Inositol 1,3,4,5,6-pentakisphosphate 2-kinase (IP5 2-K)3 is a key enzyme of higher inositol phosphate (inositide, IP) metabolism. IP5 2-K is present in yeast to mammals and catalyzes the synthesis of phytic acid (inositol hexakisphosphate or IP6) from IP5 and ATP. Mouse IP5 2-K folds in two lobes, N- and C-terminal lobes, connected by a hinge, thereby conserving the general fold scheme of PKs and IPKs, and in a similar way, both lobes coordinate the nucleotide between them. The CIP lobe represents more than half of the protein and is specific to IP5 2-K enzymes.

We have solved the structure of Mus musculus IP5 2-K (mIP5 2-K) at 2.4 Å resolution from a truncated form lacking the 21 C-terminal residues (ΔC-mIP5 2-K). In addition, we present two different crystal forms, including one or two molecules in the asymmetric unit, respectively, the first showing much better resolution (2.4 versus 3.2 Å). Unexpectedly, the formation of the ternary complex (mIP5 2-K + IP5 + ATP) was achieved by protein incubation with IP6 and ADP. The triphosphate moiety is tightly bound to the N-lobe of the enzyme through polar interactions and to the C-lobe through two magnesium ions. Regarding the inositide substrate, IP5 is tightly bound to the enzyme through its five phosphates. Residues Lys-138 and Asp-400 make direct interaction with Pγ and/or the nucleophile 2-OH. The distance between the 2-OH and Pγ oxygen is 3.2 Å suggesting an in-line transference mechanism probably in agreement with an associative mechanism. Pγ is oriented through a magnesium ion (Mg1) coordinated to Asp-437 and to Asp-439 in a second sphere. Asp-437 also coordinates a second magnesium ion (Mg2) together with Ser-402 through a water molecule. The Zn1 site is formed by residues from two CIP lobe elements: Cys-159, Cys-162, and Cys-181 from CIP-I and Cys-291 from CIP-II.

> GEFMEEGKMDENEWSYHGEGNKSLVVAHAQRCVVLRFLKFPPNKKKTSEEILQHLQNIVDFGKNVMKDFLGENYVHCGEVVQLPLEFVKQLCLKIQCERPESRCDKDLDTFSGYAMCLPNLTRLQTFHFAEHRPILCVEIKPKCGFIPFSNDVTHEMKHKVCRYCMHQHLKVATGKWKKISKYCPLDLYSGNKQRMHFALRSLLQETQNNLRIFKNGELIYGCGDARSPVADLKELAHHLKPFFFPSNGLASGPHCTKAVIRELVHVITRVLLSSSEKARAGALRLGLQGPRVCEASPFSRSLHNQGKNTSEHSGLPKGCLLYKTLQVQMLDQLDIEGLYPLYKRVEQYLEEFPEERKTLQIDGPYDEVFYQKLLDLSTEDDGTVAFALTKVQQYRVAMTAKDCSIMIALSPCLQGTSSDQRPVIPSSRSRLAFSVSVLDLDLKPYESIPHQYKLDSKIVNYYSKTVHAKD> MAAFGILSYEHRPLKRPRLGPPDVYPQDPKQKEDELTALNVKQGFNNQPAVSGDEHGSAKNVSFNPAKISSNFSSIIAEKLRCNTLPDTGRRKPQVNQKDNFWLVTARSQSAINTWFTDLAGTKPLTQLAKKVPIFSKKEEVFGYLAKYTVPVMRAAWLIKMTCAYYAAISETKVKKRHVDPFMEWTQIITKYLWEQLQKMAEYYRPGPAGSGGCGSTIGPLPHDVEVAIRQWDYTEKLAMFMFQDGMLDRHEFLTWVLECFEKIRPGEDELLKLLLPLLLRYSGEFVQSAYLSRRLAYFCTRRLALQLDGVSSHSSHVISAQSTSTLPTTPAPQPPTSSTPSTPFSDLLMCPQHRPLVFGLSCILQTILLCCPSALVWHYSLTDSRIKTGSPLDHLPIAPSNLPMPEGNSAFTQQVRAKLREIEQQIKERGQAVEVRWSFDKCQEATAGFTIGRVLHTLEVLDSHSFERSDFSNSLDSLCNRIFGLGPSKDGHEISSDDDAVVSLLCEWAVSCKRSGRHRAMVVAKLLEKRQAEIEAERCGESEAADEKGSIASGSLSAPSAPIFQDVLLQFLDTQAPMLTDPRSESERVEFFNLVLLFCELIRHDVFSHNMYTCTLISRGDLAFGAPGPRPPSPFDDPADDPEHKEAEGSSSSKLEDPGLSESMDIDPSSSVLFE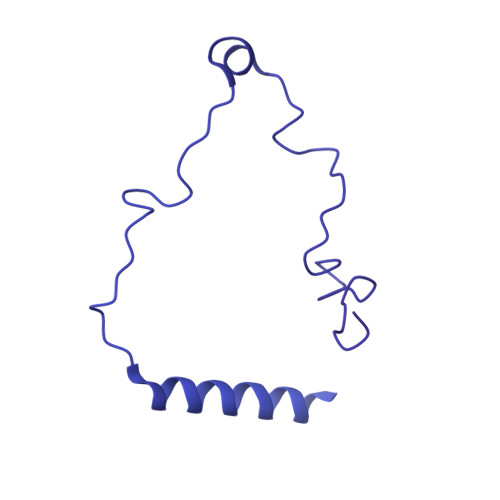DMEKPDFSLFSPTMPCEGKGSPSPEKPDVEKEVKPPPKEKIEGTLGVLYDQPRHVQYATHFPIPQEESCSHECNQRLVVLFGVGKQRDDARHAIKKITKDILKVLNRKGTAETDQLAPIVPLNPGDLTFLGGEDGQKRRRNRPEAFPTAEDIFAKFQHLSHYDQHQVTAQVSRNVLEQITSFALGMSYHLPLVQHVQFIFDLMEYSLSISGLIDFAIQLLNELSVVEAELLLKSSDLVGSYTTSLCLCIVAVLRHYHACLILNQDQMAQVFEGLCGVVKHGMNRSDGSSAERCILAYLYDLYTSCSHLKNKFGELFSDFCSKVKNTIYCNVEPSESNMRWAPEFMIDTLENPAAHTFTYTGLGKSLSENPANRYSFVCNALMHVCVGHHDPDRVNDIAILCAELTGYCKSLSAEWLGVLKALCCSSNNGTCGFNDLLCNVDVSDLSFHDSLATFVAILIARQCLLLEDLIRCAAIPSLLNAACSEQDSEPGARLTCRILLHLFKTPQLNPCQSDGNKPTVGIRSSCDRHLLAASQNRIVDGAVFAVLKAVFVLGDAELKGSGFTVTGGTEELPEEEGGGGSGGRRQGGRNISVETASLDVYAKYVLRSICQQEWVGERCLKSLCEDSNDLQDPVLSSAQAQRLMQLICYPHRLLDNEDGENPQRQRIKRILQNLDQWTMRQSSLELQLMIKQTPNNEMNSLLENIAKATIEVFQQSAETGSSSGSTASNMPSSSKTKPVLSSLERSGVWLVAPLIAKLPTSVQGHVLKAAGEELEKGQHLGSSSRKERDRQKQKSMSLLSQQPFLSLVLTCLKGQDEQREGLLTSLYSQVHQIVNNWRDDQYLDDCKPKQLMHEALKLRLNLVGGMFDTVQRSTQQTTEWAMLLLEIIISGTVDMQSNNELFTTVLDMLSVLINGTLAADMSSISQGSMEENKRAYMNLAKKLQKELGERQSDSLEKVRQLLPLPKQTRDVITCEPQGSLIDTKGNKIAGFDSIFKKEGLQVSTKQKISPWDLFEGLKPSAPLSWGWFGTVRVDRRVARGEEQQRLLLYHTHLRPRPRAYYLEPLPLPPEDEEPPAPTLLEPEKKAPEPPKTDKPGAAPPSTEERKKKSTKGKKRSQPATKTEDYGMGPGRSGPYGVTVPPDLLHHPNPGSITHLNYRQGSIGLYTQNQPLPAGGPRVDPYRPVRLPMQKLPTRPTYPGVLPTTMTGVMGLEPSSYKTSVYRQQQPAVPQGQRLRQQLQQSQGMLGQSSVHQMTPSSSYGLQTSQGYTPYVSHVGLQQHTGPAGTMVPPSYSSQPYQSTHPSTNPTLVDPTRHLQQRPSGYVHQQAPTYGHGLTSTQRFSHQTLQQTPMISTMTPMSAQGVQAGVRSTAILPEQQQQQQQQQQQQQQQQQQQQQQQQQQYHIRQQQQQQILRQQQQQQQQQQQQQQQQQQQQQQQQQQHQQQQQQQAAPPQPQPQSQPQFQRQGLQQTQQQQQTAALVRQLQQQLSNTQPQPSTNIFGRY> MLGNMNVFMAVLGII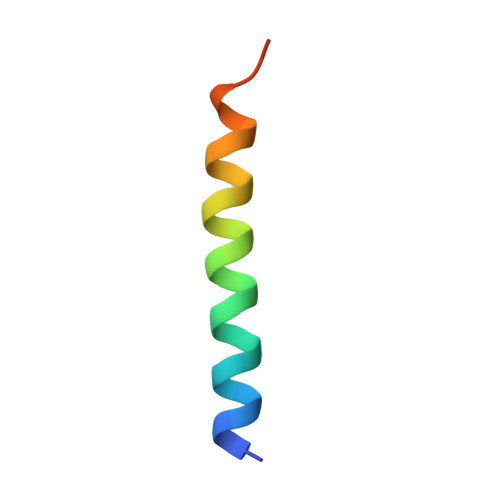LFSGFLAAYFSHKWDD> MPKEKPHVNIVFIGHVDHGKSTTIGRLLYDTGNIPETIIKKFEEMGEKGKSFKFAWVMDRLKEERERGITID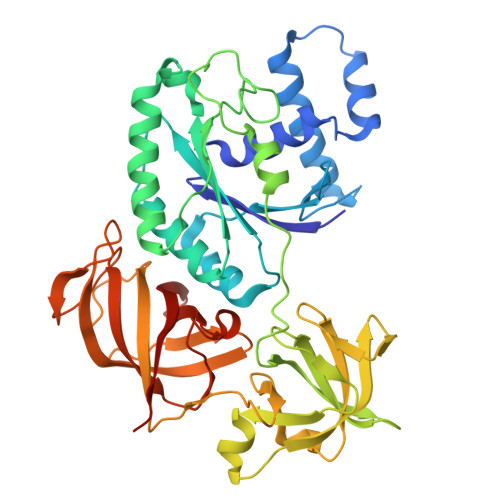VAHTKFETPHRYITIIDAPGHRDFVKNMITGASQADAAVLVVAATDGVMPQTKEHAFLARTLGIKHIIVTINKMDMVNYDQKVFEKVKAQVEKLLKTLGYKDFPVIPTSAWNGDNVVKKSDKMPWYNGPTLIEALDQIPEPEKPIDKPLRIPIQDVYSIKGVGTVPVGRVETGKLKVGDVVIFEPASTIFHKPIQGEVKSIEMHHEPLQEALPGDNIGFNVRGVSKNDIKRGDVAGHTDKPPTVVRTKDTFKAQIIVLNHPTAITVGYSPVLHAHTAQIPVRFEQILAKVDPRTGNIVEENPQFIKTGDSAIVVLRPMKPVVLEPVKEIPQLGRFAIRDMGMTIAAGMVISIQKGEHHHHHH> MAYAEWIAVKVVVSKSIGTVGIRNATLQWGKFYRYTNKDDEISTEEVSSM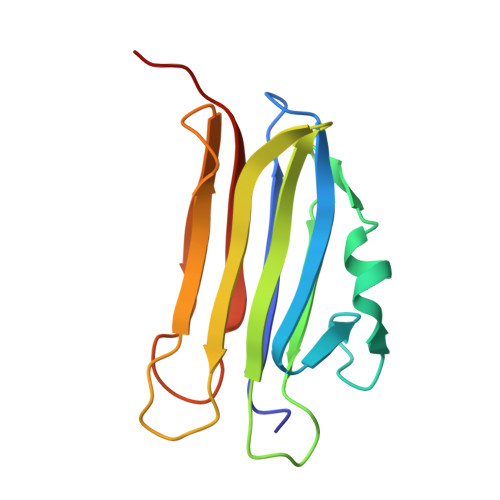NVQAGSPQWIASCGRENASSGTQGSFDCYDGNTKMGTFSWDDPWKSGATNTWSFTPASADYAGITSGGNATGTDIGEVTLTLGRFSENLYF F-spondin is a multi-domain extracellular matrix (ECM) protein and a contact-repellent molecule that directs axon outgrowth and cell migration during development. F-spondin is an extracellular matrix (ECM) protein with multiple domains, including an N-terminal domain (reelin_N domain), an F-spondin (FS) domain and six thrombospondin type 1 repeats (TSRs). The reelin_N domain and the F-spondin domain (FS domain) comprise a proteolytic fragment that interacts with the cell membrane and guides the projection of commissural axons to floor plate. In this paper, we present the crystal structure of human F-spondin FS domain.

The core of the FS domain has an 8-stranded β-sandwich fold, with strands β4, β1, β8, and β7 forming one β-sheet and strands β3, β2, β5 and β6 forming the other sheet. The first major variation of the FS domain, as compared to a common C2 domain, is its long linker (38 amino acids) between β2 and β3 strands, which actually forms two anti-parallel α-helices, packed against the β3/β2/β5/β6 sheet. The second variation is its long linker (51 amino acids) between the β7 and β8 strands. The three consecutive cysteines (C199, C200 and C202) before the β1 strands form three disulfide bonds with C336 and C340 from the β6-β7 loop, and C415 after the β8 strand at the C-terminal region, respectively. None of these disulfide bonds is located within the core of the β-sandwich domain. They are all at the bottom of the FS domain and are associated with N- and C-termini, especially the N-terminus, where they seem to help define and stabilize the globular FS domain. There is one N-linked glycosylation site (N214) at the end of the β1 strand in the FS domain. The common pentasaccharide core of the linked glycans is visible in the electron densities. Associated with the short strands at the top of the FS domain, there is a solvent-accessible Ca2+-binding site, formed from D325 (from β5-β6 loop), D354 (from β7' short strand) and D358 (right after β7' short strand). All three aspartic acids are from the two highly conserved and characteristic FS domain "repeats", P322SPDW and D354AGTD (in F-spondin). Both D325 and D354 interact with the Ca2+ ion as bidentate ligands involving both carboxyl groups with bond distances of 2.49 Å/2.53 Å and 2.38 Å/2.46 Å, respectively. The homology of its core structure to a common Ca2+- and lipid-binding C2 domain suggests that the F-spondin FS domain may be responsible for part of the membrane targeting of F-spondin in its regulation of axon development.

> RSPWPGVTDKPILDCCACGTAKYRLTFYGNWSEKTHPKDYPRRANHWSAIIGGSHSKNYVLWEYGGYASEGVKQVAELGSPVKMEEEIRQQSDEVLTVIKAKAQWPAWQPLNVRAAPSAEFSVDRTRHLMSFLTMMGPSPDWNVGLSAEDLCTKECGWVQKVVQDLIPWDAGTDSGVTYESPNKPTIPQEKIRPLTSLDHPQSPFYDPEGGSITQVARVVIERIARKGEQCNIVPDNVDDIVADLAPEEKTGHHHHHH>MAATSRPERVWPDGVIPFVIGGNFTGSQRAVFRQAMRHWEKHTCVTFLERTDEDSYIVFTYRPCGCCSYVGRRGGGPQAISIGKNCDKFGIVVHELGHVVGFWHEHTRPDRDRHVSIVRENIQPGQEYNFLKMEPQEVESLGETYDFDSIMHYARNTFSRGIFLDTIVPKYEVNGVKPPIGQRTRLSKGDIAQARKLYKCPA[2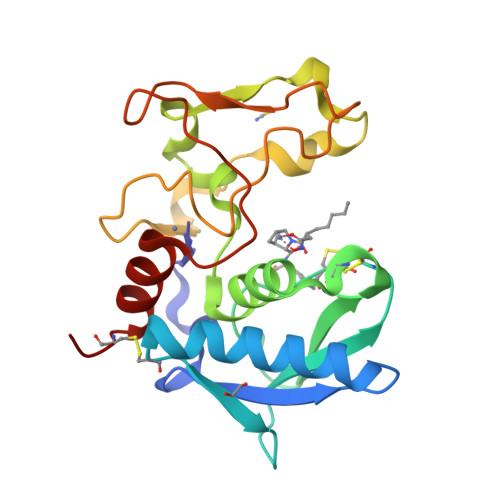x]> MRGSHHHHHHGSIWEWKEAHFQDAFSSFQAMYAKSYATEEEK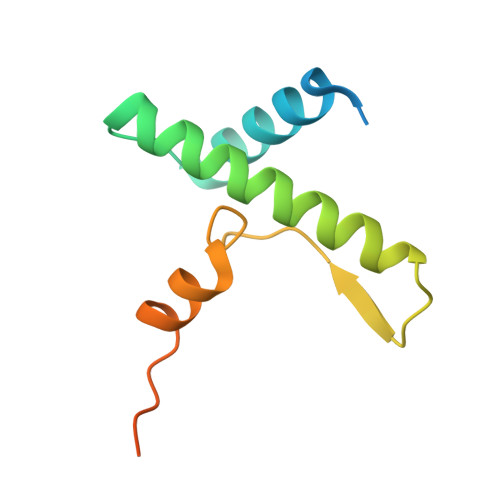QRRYAIFKNNLVYIHTHNQQGYSYSLKMNHFGDLSRDEFRRKYLGFKKSRNLKSHHLGVATELL Transmembrane protein 2 (TMEM2) is a cell surface protein that has been reported to degrade HA into ~5 kDa fragments and play an essential role in systemic HA turnover. Recently, two homologous proteins that are not members of the HYAL family have been implicated in extracellular HA degradation: CEMIP (cell migration-inducing and hyaluronan-binding protein, also called KIAA1199 or HYBID) and TMEM2 (transmembrane protein 2). The two proteins share the same domain structure (see below) but differ in one important respect: CEMIP is a secreted protein, whereas TMEM2 is a type II transmembrane protein in the plasma membrane 3 . Subsequent studies showed that TMEM2 is essential for systemic HA turnover 6 and that it regulates cell adhesion and migration via HA degradation at focal adhesion sites 7 .

We expressed the soluble ectodomain of human TMEM2 (residues 106-1383; sTMEM2) with a N-terminal hexahistidine tag in Expi293 cells. We collected a high-redundancy X-ray diffraction data set (deposited in the PDB, see Underlying data) to 3.5 Å resolution and solved the structure by molecular replacement using the AlphaFold model of TMEM2 9 . Nearly the entire ectodomain (residues 112-1381) is resolved in the crystal structure, which matches the AlphaFold model with a root-mean-square (r.m.s.) deviation of only 1.1 Å (1270 Cα atoms). The sTMEM2 structure is built around a 70 Å-long right-handed parallel β-helix that starts at the N terminus. A small β-sandwich and a larger lectin-like domain (26% sequence identity to the N-terminal domain of protein O-linked-mannose β-1,2-N-acetylglucosaminyltransferase 1 (POMGNT1) 20 ) are inserted into the β-helix after three complete turns without disrupting its regular structure. The β-helix is followed by a large β-sandwich that is not closely related to any other known structure (termed domain X). The polypeptide chain then runs halfway down the β-helix before forming a second lectin-like domain (20% identity to POMGNT1) and, finally, a C terminal helix. The majority of active sites are located roughly in the middle of the β-helix, which in sTMEM2 is obstructed by two long loops, made up of residues 627-662 and 733-756. The three key sugar-binding residues of POMGNT1 are conserved in TMEM2, suggesting that lectin-like domain 1 may bind carbohydrates. We found that pure, crystallisable, soluble TMEM2 has no detectable hyaluronidase activity.

> APLVHHHHHHALDENLYFQGALAKYAPDENCPDQNPRLRNWDPGQDSAKQVVIKEGDMLRLTSDATVHSIVIQDGGLLVFGDNKDGSRNITLRTHYILIQDGGALHIGAEKCRYKSKATITLYGKSDEGESMPTFGKKFIGVEAGGTLELHGARKASWTLLARTLNSSGLPFGSYTFEKDFSRGLNVRVIDQDTAKILESERFDTHEYRNESRRLQEFLRFQDPGRIVAIAVGDSAAKSLLQGTIQMIQERLGSELIQGLGYRQAWALVGVIDGGSTSCNESVRNYENHSSGGKALAQREFYTVDGQKFSVTAYSEWIEGVSLSGFRVEVVDGVKLNLLDDVSSWKPGDQIVVASTDYSMYQAEEFTLLPCSECSHFQVKVKETPQFLHMGEIIDGVDMRAEVGILTRNIVIQGEVEDSCYAENQCQFFDYDTFGGHIMIMKNFTSVHLSYVELKHMGQQQMGRYPVHFHLCGDVDYKGGYRHATFVDGLSIHHSFSRCITVHGTNGLLIKDTIGFDTLGHCFFLEDGIEQRNTLFHNLGLLTKPGTLLPTDRNNSMCTTMRDKVFGNYIPVPATDCMAVSTFWIAHPNNNLINNAAAGSQDAGIWYLFHKEPTGESSGLQLLAKPELTPLGIFYNNRVHSNFKAGLFIDKGVKTTNSSAADPREYLCLDNSARFRPHQDANPEKPRVAALIDRLIAFKNNDNGAWVRGGDIIVQNSAFADNGIGLTFASDGSFPSDEGSSQEVSESLFVGESRNYGFQGGQNKYVGTGGIDQKPRTLPRNRTFPIRGFQIYDGPIHLTRSTFKKYVPTPDRYSSAIGFLMKNSWQITPRNNISLVKFGPHVSLNVFFGKPGPWFEDCEMDGDKNSIFHDIDGSVTGYKDAYVGRMDNYLIRHPSCVNVSKWNAVICSGTYAQVYVQTWSTQNLSMTITRDEYPSNPMVLRGINQKAAFPQYQPVVMLEKGYTIHWNGPAPRTTFLYLVNFNKNDWIRVGLCYPSNTSFQVTFGYLQRQNGSLSKIEEYEPVHSLEELQRKQSERKFYFDSSTGLLFLYLKAKSHRHGHSYCSSQGCERVKIQAATDSKDISNCMAKAYPQYYRKPSVVKRMPAMLTGLCQGCGTRQVVFTSDPHKSYLPVQFQSPDKAETQRGDPSVISVNGTDFTFRSAGVLLLVVDPCSVPFRLTEKTVFPLADVSRIEEYLKTGIPPRSIVLLSTRGEIKQLNISHLLVPLGLAKPAHLYDKGSTIFLGFSGNFKPSWTKLFTSPAGQGLGVLEQFIPLQLDEYGCPRATTVRRRDLELLKQASKAH>[4x]MSATLPDMDTLRERLLAGDRAALARAITLAESRRADHRAAVRDLIDAVLPQT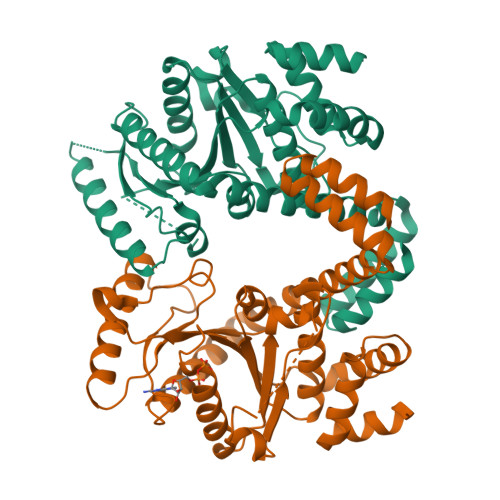GRAIRVGITGVPGVGKSTTIDALGSLLTAAGHKVAVLAVDPSSTRTGGSILGDKTRMARLAIDRNAFIRPSPSSGTLGGVAAKTRETMLLCEAAGFDVILVETVGVGQSETAVADLTDFFLVLMLPGAGDELQGIKKGIFELADMIAVNKADDGDGERRASAAASEYRAALHILTPPSATWTPPVVTISGLHGKGLDSLWSRIEDHRSKLTATGEIAGKRREQDVKWMWALVHERLHQRLVGSAEVRQATAEAERAVAGGEHSPAAGADAIATLIGLLEHHHHHH> MKFTPSIVIDAPQYYVDHFNGKYNVDKCVILRDLQLETDSESMPSSLKHLTKPTHILDLTNNDLIMIPDLSRRDDIHTLLLGRNNIVEVDGR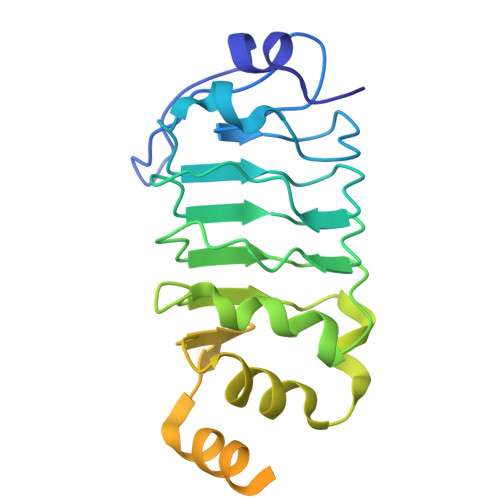LLPMNVQNLTLSNNSIRRFEDLQRLRRAPRTLKNLTLIGNQVCHLANYREHVLRLVPHLETLDFQNVTAEERKSAMSFPRQADGDTLGPVNTAIRDNGSRDKTMEIMNLVVSKMTVERRNELKKQLAEATSLEEIARLEKLLSGGV>[2x]MIDYTAAGFTLLQGAHLYAPEDRGICDVLVANGKIIAVASNIPSDIVPNCTVVDLSGQILCPGFI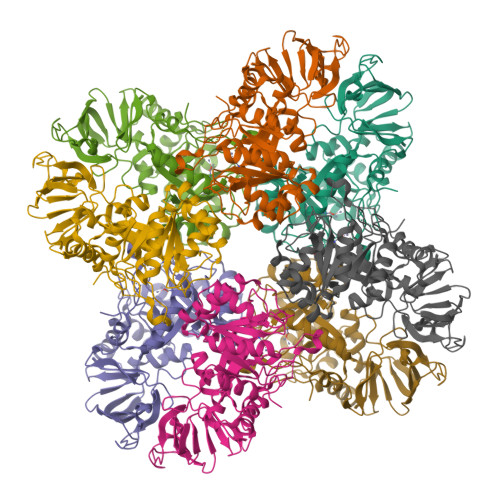DQHVHLIGGGGEAGPTTRTPEVALSRLTEAGVTSVVGLLGTDSISRHPESLLAKTRALNEEGISAWMLTGAFHVPSRTITGSVEKDVAIIDRVIGVKCAISDHRSAAPDVYHLANMAAESRVGGLLGGKPGVTVFHMGDSKKALQPIYDLLENCDVPISKLLPTHVNRNVPLFEQALEFARKGGTIDITSSIDEPVAPAEGIARAVQAGIPLARVTLSSDGNGSQPFFDDEGNLTHIGVAGFETLLETVQVLVKDYDFSISDALRPLTSSVAGFLNLTGKGEILPGNDADLLVMTPELRIEQVYARGKLMVKDGKACVKGTFETA>[2x]QEGDPEAGAKAFNQCQTCHVIVDDSGTTIAGRNAKTGPNLYGVVGRTAGTQADFKGYGEGMKEAGAKGLAWDEEHFVQYVQDPTKFLKEYTGDAKAKGKMTFKLKKEADAHN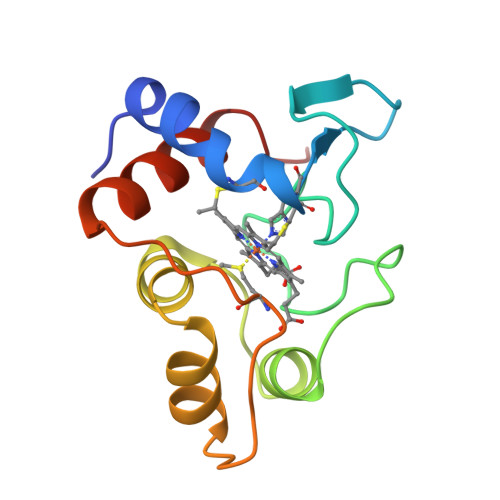IWAYLQQVAVRP Serum amyloid P component (SAP) is a normal plasma glycoprotein that recognizes and binds to amyloid fibres in a calcium-dependent fashion wherever these are deposited in tissues. In summary, the structure of SAP is comprised of five identical 204-residue subunits associated in a ring 95 Å in diameter and 35 Å deep, with radial symmetry creating a central pore 20 Å wide. Each protomer consists of 15 β-strands (labelled A to O from the N-terminus to the C-terminus) arranged in two large β-sheets in the form of a flattened β-barrel with jelly-roll topology. The β-sheets are held nearly perpendicular to the radial symmetry, creating two separate and distinct faces: the A face, which contains five α-helices, and the opposing B face, which contains five double metal-binding sites formed by the coordination of six localized protein residues.

Crystals of the SAP–CPHPC complex grown in the presence of calcium ions and a tenfold molar excess of CPHPC at 4°C have been reported previously. The crystals contained a large tetragonal unit cell containing approximately 83% solvent and ten SAP sub­units in the asymmetric unit. The crystals did not tolerate removal from the cold room prior to vitrification, and not unexpectedly their diffraction was relatively weak (limited to 3.2 Å resolution). Radiation damage caused rupture of some disulfide bridges, but the conformational effects were local. This structure was determined using molecular replacement, and here we have revisited the refinement in the light of developments in procedures for medium-resolution data. Structural studies of the SAP–CPHPC complex by X-ray diffraction at medium resolution (3.2 Å) showed that in addition to a carboxylate interaction with the calcium site of SAP, the pyrrolidine ring of the d-proline constituents of CPHPC bound into a hydrophobic pocket formed by the side chains of Tyr74, Tyr64 and Leu62. The approach of each d-proline head group to the opposing sites of the in-register twofold axis-related pairs of subunits of the SAP decamer appeared to be facilitated by a kinked rotamer at the centre of the alkyl linker. Model building of the CPHPC ligand into the tenfold NCS averaged electron density of the lower resolution SAP–calcium map did not clearly establish whether the peptide bond preceding the proline ring was in the cis or the trans form, and in the deposited coordinates both cis and trans isomers were included for each ligand. Five molecules of the bivalent ligand cross-link and stabilize pairs of SAP molecules, forming a decameric complex that is rapidly cleared from the circulation by the liver.

>HTDLSGKVFVFPRESVTDHVNLITPLEKPLQNFTLCFRAYSDLSRAYSLFSYNTQGRDNELLVYKERVGEYSLYIGRHKVTSKVIEKFPAPVHICVSWESSSGIAEFWINGTPLVKKGLRQGYFVEAQPKIVLGQEQDSYGGKFDRSQSFVGEIGDLYMWDSVLPPENILSAYQGTPLPANILDWQALNYEIRGYVIIKPLVWV[10x]> GSHMTNPQFAGHPFGTTVTAETLRNTFAPLTQWEDKYRQLIMLGKQLPALPDELKAQAKEIAGCENRVWLGYTVAENGKMHFFGDSEGRIVRGLLAVLLTAVEGKTAAE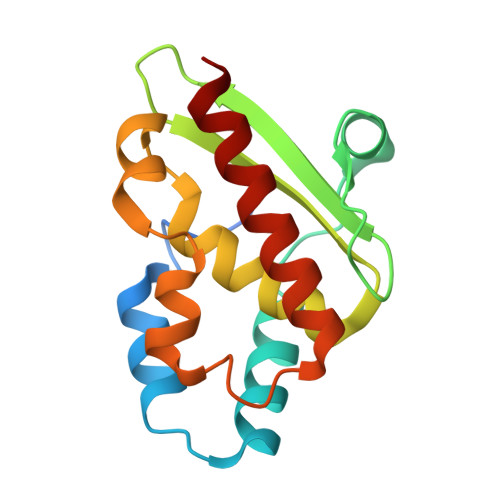LQAQSPLALFDELGLRAQLSASRSQGLNALSEAIIAAAKQV> LDAFSKVITSADGKAAYVGGADLQALKKFVSDGNKRMDAVNAIVSNASCIVSDAVSGMVCENPSLIAPNGGVYSNRKMAA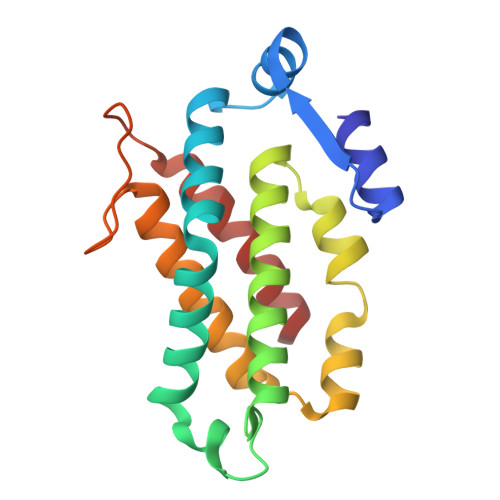CLRDAEIILRYVSYSLLSGDSSVLEDRCLNGLKETYSSLGVPAAGNARAVAIMKATVNSFINNTAQQKKLSVPSGDCSALASEAGGYFDKVTSAIA>[2x]MNIMLTGA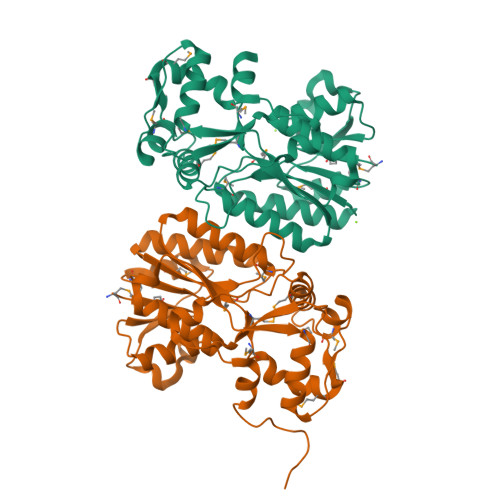TGHLGTHITNQAIANHIDHFHIGVRNVEKVPDDWRGKVSVRQLDYFNQESMVEAFKGMDTVVFIPSIIHPSFKRIPEVENLVYAAKQSGVAHIIFIGYYADQHNNPFHMSPYFGYASRLLSTSGIDYTYVRMAMYMDPLKPYLPELMNMHKLIYPAGDGRINYITRNDIARGVIAIIKNPDTWGKRYLLSGYSYDMKELAAILSEASGTEIKYEPVSLETFAEMYDEPKGFGALLASMYHAGARGLLDQESNDFKQLVNDQPQTLQSFLQENILEHHHHHH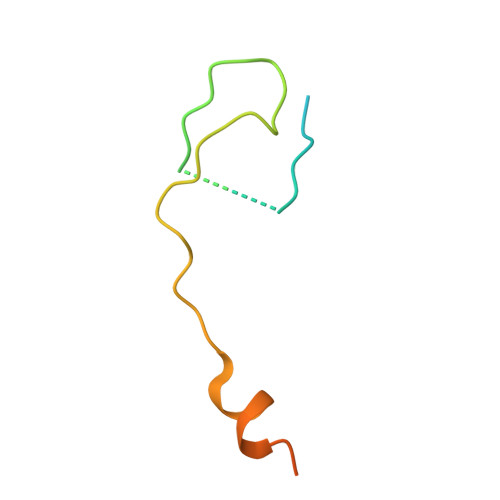> MGSQVSTQRSGSHENSNSASEGSTINYTTINYYKDAYAASAGRQDMSQDPKKFTDPVMDVIHEMAPPLK> SEESELYHAQIHLYKHVYNFVSSMALKSAMELGIADAIHNHGKPMTLSELASSLKLHPSKVNILHRFLRLLTHNGFFAKTIVKGKEGDEEEEIA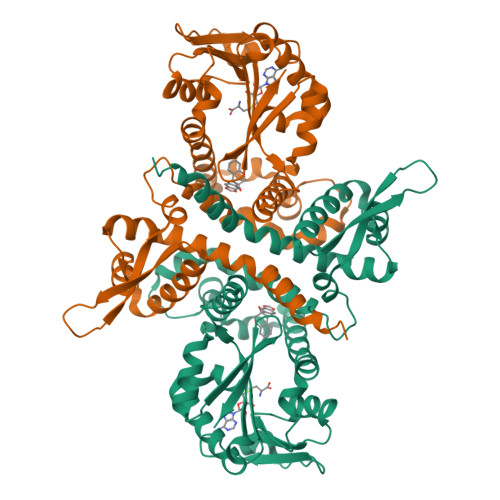YSLTPPSKLLISGKPTCLSSIVKGALHPSSLDMWSSSKKWFNEDKEQTLFECATGESFWDFLNKDSESSTLSMFQDAMASDSRMFKLVLQENKRVFEGLESLVDVGGGTGGVTKLIHEIFPHLKCTVFDQPQVVGNLTGNENLNFVGGDMFKSIPSADAVLLKWVLHDWNDEQSLKILKNSKEAISHKGKDGKVIIIDISIDETSDDRGLTELQLDYDLVMLTMFLGKERTKQEWEKLIYDAGFSSYKITPISGFKSLIEVYP Staufen proteins bind structured mRNA motifs through dsRNA-binding domains (dsRBD) and are involved in mRNA localization in Drosophila and mammals. Members of the Stau protein family share a common domain organization, consisting of four to five copies of the dsRNA-binding domain (dsRBD) separated by linkers that are predicted to be unstructured. Similarly, a stem of 19 bp is required for the binding of human Stau1 (hStau1) to the 3ʹUTR of ADP-Ribosylation Factor 1 (ARF1) mRNA. To understand how Stau recognizes its target RNAs, we determined the crystal structure of the minimal RNA-binding region of hStau1, consisting of dsRBDs 3 and 4, in complex with the 19 bp SBS from ARF1 mRNA.

The structure, at 2.9 Å resolution, shows that the tandem dsRBDs of hStau1 recognize A-form RNA, mainly through electrostatic interactions with the RNA backbone. A difference Fourier map, calculated using phases from a derivative complex containing SeMet-substituted hStau1 dsRBD3-4, showed peaks at the expected Met positions in all three domains (M181 and M213 for dsRBD3, and M321 and M348 for dsRBD4). This allowed the validation of the correct placement and assignment of the domains and confirmed the presence of two dsRBD3 domains (designated dsRBD3A and dsRBD3B), but only one dsRBD4 associated to one molecule of RNA. DsRBD3B is bound on the opposite side of the RNA molecule, in an antiparallel orientation to dsRBD3A, whereas the second dsRBD4 is missing and likely to be unbound and disordered, possibly because of steric clashes with the other bound dsRBDs. DsRBD3A and dsRBD4 bind to the RNA next to each other, sharing a heterodimerization interface of 273 Å2 (5.1% of their total surface) (calculated with PISA; Krissinel & Henrick, 2007), which engages strand β1 of dsRBD3A and helix α2 of dsRBD4. Region 1, consisting of helix α1, contacts the minor groove of the dsRNA; region 2, formed by the loop between strands β1 and β2, interacts with the adjacent minor groove surface; region 3, comprising a patch of basic residues at the N-terminal tip of helix α2, inserts in the intervening major groove. Both dsRBD3 molecules in our structure engage all three regions in RNA binding. Conversely, dsRBD4 primarily uses regions 1 and 3 for binding, whereas the β1–β2 loop in region 2 is partially unstructured and does not engage in close interactions with the RNA. In addition to the interactions with the sugar–phosphate backbone, both domains of hStau1 in our structure directly contact RNA bases in the minor groove of ARF1 SBS. Within the β1–β2 loop of dsRBD3A, the backbone oxygen of P211 establishes a base-specific contact with the N2 group of G77; the same loop is reoriented in dsRBD3B and points toward the minor groove of the symmetry-related RNA molecule without engaging in base-directed contacts, whereas in dsRBD4, the β1–β2 loop is not in close contact with the minor groove.

>[3x]GHMNKSEISQVFEIALKRNLPVNFEVARESGPPHMKNFVTKVSVGEFVGEGEGKSKKISKKNAAIAVLEELKKLPPLPAVERVKPRIKKKTKPIVKPQTSPEYGQGINPISRLAQIQQAKKEKEPEYTLLTERGLPRRREFVMQVKVGNHTAEGTGTNKKVAKRNAAENMLEILGFKVPQRQ> GAMDVLSEKIWDYHNKVSQTDEMLQRKLHLRDMLYTAISPVFPLSGLYVVGSSLNGFGNNSSDMDLCLMITNKDLDQKNDAVVVLNLILSTLQYEKFVESQKLILAKVPILRINFAAPFDDITVALNANNSVAIRNTHLLCYYSSYDW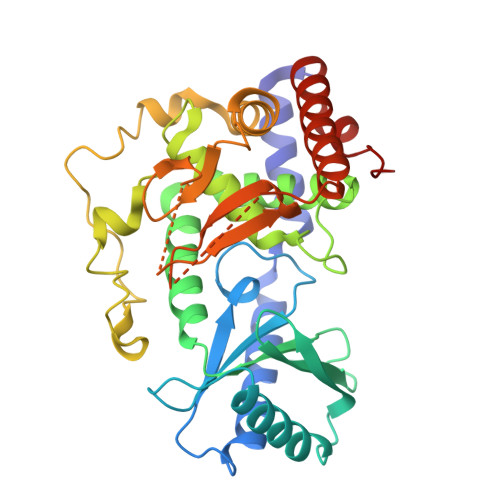RVRPLVSVVKEWAKRKGINDANKSSFTSYSLVLMVIHFLQCGPTKVLPNLQQSYPNRFSNKVDVRTLNVTMALEEVADDIDQSLSEKTTLGELLIGFLDYYANEFNYDRDAISIRQGRRVERASISNPHFWRSQWRCVCIEEPFTNSNTAHSIYDEMVFEAIKKAFREAHGELQHNHDLDKLMECEPIKA>MGHHHHHHSHSHMELYECIQDIFGGLKNPSVKDLATSLKQIPNAAKLSQPYIKEPDQYAYGRNAIYRNNELEIIVINIPPNKETTVHDHGQSIGCAMVLEGKLLNSIYRSTGEHAELSNSYFVHEGECLISTKGLIHKMSNPTSERM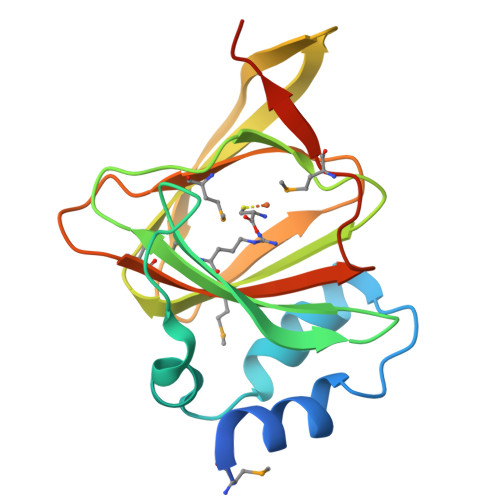VSLHVYSPPLEDMTVFEEQKEVLENS[2x]>[4x]MFLAPWIERRLRYHPTIELPDDTRGHILIFGIDPITRT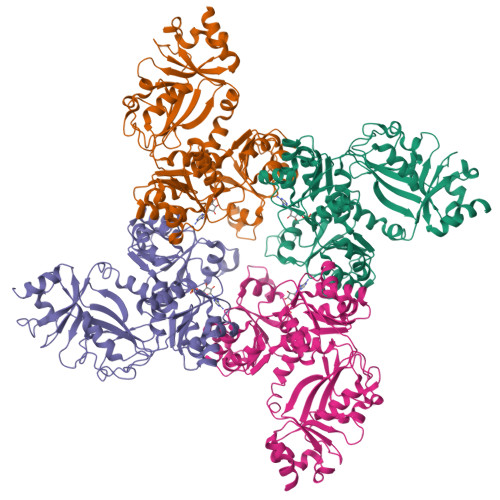LIRKLESRNHLFVVVTDNYDQALHLEEQEGFKVVYGSPTDAHVLAGLRVAAARSIIANLSDPDNANLCLTVRSLCQTPIIAVVKEPVHGELLRLAGANQVVPLTRILGRYLGIRATTCGALAHILDSFGNLQIAELPVHGTPFAGKTIGESGIRQRTGLSIIGVWERGSLTTPQRETVLTEQSLLVLAGTKSQLAALEYLIGEAPEDELIFIIGHGRIGCAAAAFLDRKPVPFILIDRQESPVCNDHVVVYGDATVGQTLRQAGIDRASGIIVTTNDDSTNIFLTLACRHLHSHIRIVARANGEENVDQLYAAGADFVVSNASVGANILGNLLEHKESAFLSEGMAVFRRPLPPAMAGKTIAETRLRPLTGCSIVAIEAPDRADILISPPPETILAEGARLILIGTSEQEKTFDQTIAARLVPR> IVGGKVCPKGECPWQVLLLVNGAQLCGGTLINTIWVVSAAHCFDKIKNWRNLIAVLGEHDLSEHDGDEQSRRVAQVIIPSTYVPGTTNHDIALLRLHQPVVLTDHVVPLCLPERTFSERTLAFVRFSLVSGWGQLLDRGATALELMVL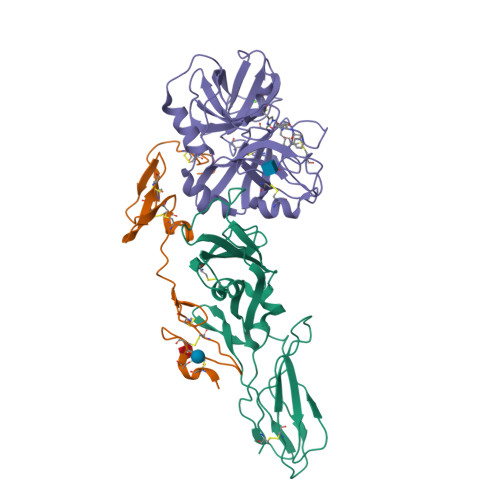NVPRLMTQDCLQQSRKVGDSPNITEYMFCAGYSDGSKDSCKGDSGGPHATHYRGTWYLTGIVSWGQGCATVGHFGVYTRVSQYIEWLQKLMRSEPRPGVLLRAPFP;> DQCASSPCQNGGSCKDQLQSYICFCLPAFEGRNCETHKDDQLICVNENGGCEQYCSDHTGTKRSCRCHEGYSLLADGVSCTPTVEYPCGKIPILE;> SGTTNTVAAYNLTWKSTNFKTILEWEPKPVNQVYTVQISTKSGDWKSKCFYTTDTECDLTDEIVKDVKQTYLARVFSYPAGNVESTGSAGEPLYENSPEFTPYLETNLGQPTIQSFEQVGTKVNVTVEDERTLVRRNNTFLSLRDVFGKDLIYTLYYWKSSSSGKKTAKTNTNEFLIDVDKGENYCFSVQAVIPSRTVNRKSTDSPVECM> MAHHHHHHMTLTFNIKVIEAKDLPKVDTFGKVDPYVQIQLGNEKCKTKVIKKSYNPVWNETFSIPVTNPKAPLNITVVDYDFI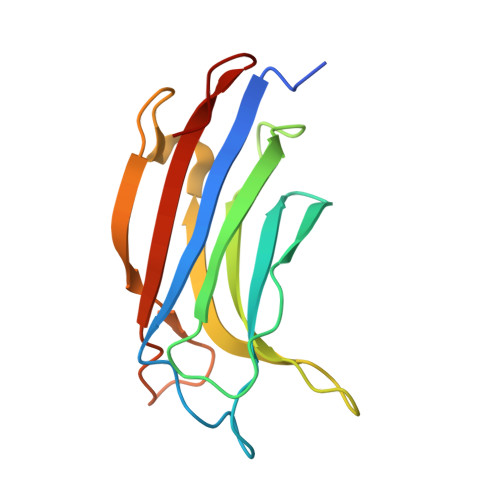GSNDAFAYIHFNQQEFNVGQVVDKWYMLNSYKAGRSAGQIHLVIHLATQNMKPFE>[2x]MGFLQGKKILITGMISERSIAYGIAKACREQGAELAFTYVVDKLEERVRKMAAELDSEL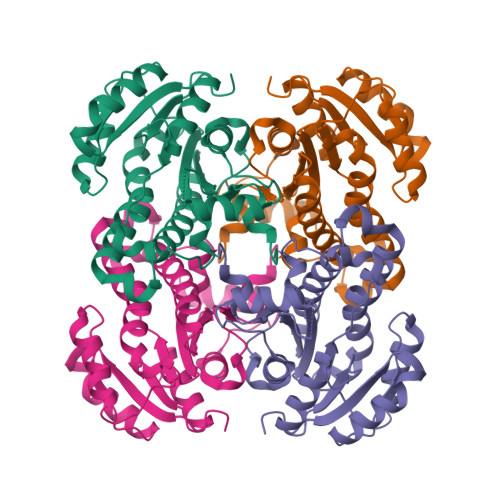VFRCDVASDDEINQVFADLGKHWDGLDGLVHSIGFAPKEALSGDFLDSISREAFNTAHEISAYSLPALAKAARPMMRGRNSAIVALSYLGAVRAIPNYNVMGMAKASLEAGIRFTAACLGKEGIRCNGISAGPIKTLAASGIADFGKLLGHVAAHNPLRRNVTIEEVGNTAAFLLSDLSSGITGEITYVDGGYSINALSTEG> SESQEAVIRDIARHLARIGDRME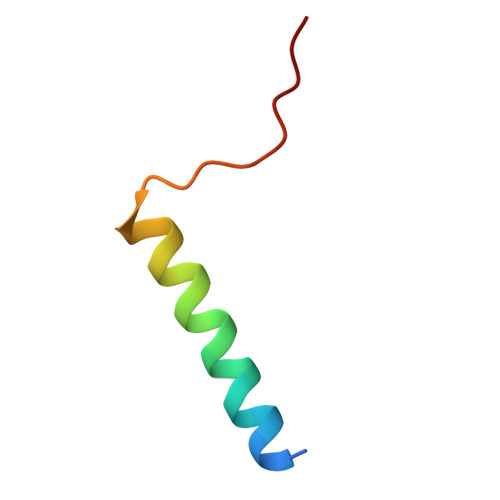YGIRPGLVDSL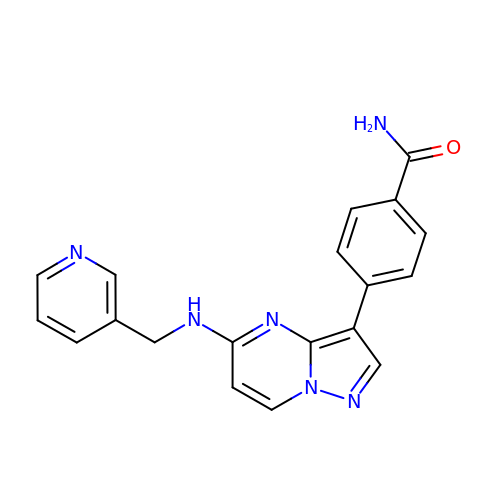4-[5-(pyridin-3-ylmethylamino)pyrazolo[1,5-a]pyrimidin-3-yl]benzamide | C19 H16 N6 O | LMGXQBQAUALFTB-UHFFFAOYSA-N>[4x]MGSQRTTAVKGERQSRVHTGNPHPTLTYDIGRVLGNGSFGVVTEARCVDTGEVVAIKKVLQDPRYKNRELDIMKELKHPNVVKLIDYFYTEMGERDSNDHNRFLNVVMEHIPETVYRVMKSFLRANQQVPFILIKLYTYQMCRALGYLHALGICHRDIKPQNLLVDSRTHVLKLCDFGSAKRLVPGEQSVSYICSRFYRAPELMLGASEYTTAIDVWSIGCVLGELLLGRPLFAGETSVDQLVKIIQILGTPSRRQMSTMNPNYTEFRFPDVKPREWKSIFASHIASTETNDPSWDQALDLLTKFLRYEPGERLLPLEALAHDFFDELRLPSTRLPSGGPLPELFTFSQLELQNMSPAAQVKCIPKGHHHHHH

Using a forward genetic approach based on transcriptome sequencing, we identified the T. gondii GSK3 (TgGSK3), a serine/threonine kinase, as the primary enzymatic target of LY2090314. TgGSK3 was identified as a fitness-conferring gene for tachyzoites, as its genetic disruption results in a fitness score of −4.1223. TgGSK3 adopts the characteristic kinase fold, divided into two sub-domains classified as the N- and C-Lobe. Overall, TgGSK3 has high sequence (54% identity) and structural conservation (r.m.s.d. of 1.67 Å) to the human ortholog, with most of the structural variation located within loops in the N-lobe (N-terminal region).

The kinase-dead Y2H screen identified TgGSK3 as its own primary interaction hub, suggesting a mechanism of homo-dimerization or multimerization. In solution, however, the recombinant TgGSK3 expressed in insect cells predominantly exists as a monomer, indicating that homo-oligomerization process does not occur spontaneously, but is instead dependent on external factors such as substrate binding, co-factors, interacting partners, or post-translational modifications. In this regard, during crystallization trials of TgGSK3 with LY2090314, an intriguing observation was made: alongside the standard crystal forms, a monoclinic crystal lattice emerged after several weeks, diffracting at lower resolution (3.0 Å) and containing four TgGSK3 subunits within the asymmetric unit. These four subunits can be reduced to two homodimers, interacting through non-crystallographic symmetry. In each dimer, TgGSK3 forms a face-to-face interaction, relying partly on the seed region identified in the yeast 2-hybrid screening, which spans most of the N-lobe. Additionally, the dimer is crosslinked by a disulfide bridge formed between the cysteine 213 of adjacent monomers. This peculiar cysteine, located on the activation loop just two residues downstream of the phosphotyrosine 211, requires significant structural rearrangements to enable bond formation with the neighboring subunit when compared to the monomeric orthorhombic crystal structure of TgGSK3. Despite these structural rearrangements, the activation loop remains in a DFG “in” conformation due to the interaction with LY2090314. While these findings may not directly translate to TgGSK3, given the distinct functional role of the two kinases, they highlight a broader role for this cysteine in regulating dimerization and activation through redox signaling. Together, the Y2H results and the monoclinic crystal structure suggest that the activation pathway of TgGSK3 in T. gondii relies on a homodimerization process, likely controlled by the conserved cysteine 213, a feature preserved across species. Converging evidence from yeast two-hybrid assays and crystallographic analyses revealed covalent dimerization of TgGSK3, mediated by a conserved cysteine residue within the activation loop.> SMVEVLADHPGELVRTDSPNFLCSVLPTHWRCNKTLPIAFKVVALGDVPDGTLVTVMAGNDENYSAELRNATA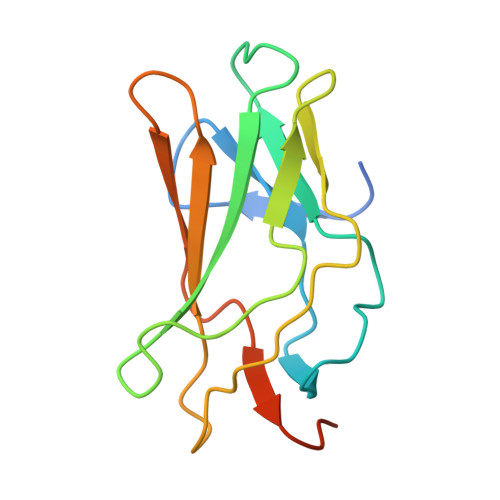AMKNQVARFNDLRFVGRSGRGKSFTLTITVFTNPPQVATYHRAIKITVDGPREPRRHRQKL>[6x]MEALGMIETRGLVALIEASDAMVKAARVKLVGVKQIGGGLCTAMVRGDVAACKAATDA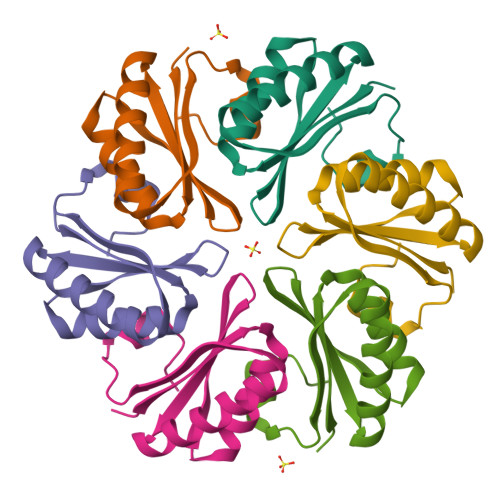GAAAAQRIGELVSVHVIPRPHGDLEEVFPIGLKGDSSNLLEHHHHHH An affordable 3D-printed, X-ray-compatible microfluidic device (3D-MiXD) is reported that allows data to be collected from protein microcrystals in a 3D flow with very high hit and indexing rates, while keeping the sample consumption low. By designing a microfluidic chip capable of centering protein microcrystals in a stable 3D liquid flow, serial synchrotron crystallographic data sets could be collected with low sample consumptions and fast collection times.

Protocols for the microcrystallization of ADC were developed in-house and are fully described in Section 2. The two different proteins microcrystallize from significantly different precipitant mixtures: PEG 6000 with NaCl for lysozyme and ammonium sulfate for ADC. Seven ADC data sets were collected at distances varying between 0 and 6 mm from the flow-focusing cross. At a constant 10:1 flow-focusing ratio between the buffer and the crystalline slurry and at a total flow rate of 550 µl h−1, this 6 mm distance is equivalent to 2.14 s of sample-travel time from the start of the flow-focusing region. The overall indexable hit rate for all ADC data sets was very high, varying between 13 and 40% of all X-ray ‘on’ images. Two final experiments were run to further elucidate the performance of these devices. Firstly, a further ADC data set was collected 3 mm downstream of the flow-focusing region [position E in Fig. 3(b)] at a buffer:sample flow-focusing ratio of 5:1, with a correlated decrease in the overall flow rate to 300 µl h−1 (compared with the previous 10:1 ratio and 550 µl h−1). The indexable hit rate did not increase under these conditions, showing that the number of hits is mostly defined by the sample concentration rather than the flow-focusing ratio or the speed of the sample inside the chip (up to 5 mm s−1). The overall X-ray dose (diffraction-weighted) was calculated with RADDOSE3D to be 74 kGy for ADC and 55 kGy for lysozyme. As expected, there was no evidence of radiation damage to the proteins during this room-temperature data collection, with both proteins showing intact disulfide bonds and carboxylate-containing side chains.

>[2x]MRGSHHHHHHGLVPRGSMIRTMLQGKLHRVKVTHADLHYEG;>XCAIDQDFLDAAGILENEAIDIWNVTNGKRFSTYAIAAERGSRIISVNGAAAHCASVGDIVIIASFVTMPDEEARTWRPNVAYFEGDNEMKRTAKAIPVQVA[2x]> MSSSIREEVHRHLGTVALMQPALHQQTHAPAPTEITHTLFRAYTRVPHDVGGEADVPIEYHEKEEEIWELNTFATCECLAWRG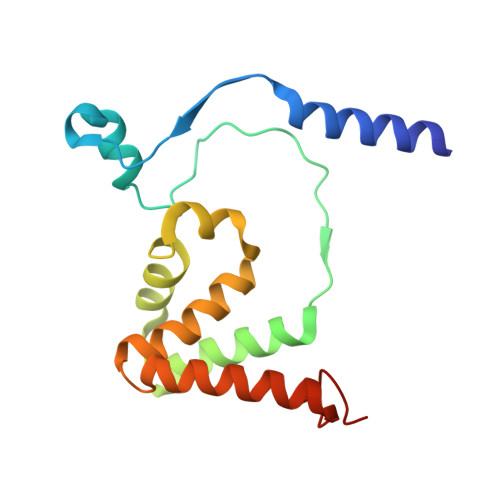VWTAEERRRKQNCDVGQTVYLGMPYYGRWLLTAARILVDKQFVTLTELHNKIVEMRERVASGQGLGEYLPPKAK> MSQLVLILGDQLSPSIAALDGVDKKQDTIVLCEVMAEASYVGHHKKKIAFIFSAMRHFAEELRGEGYRVRYTRIDDADNAGSFTGEVKRAIDDLTPSRICVTEPGEWRVRSEMDGFAGAFGIQVDIRSDRRFLSSHGEFRNWAAGRKSLT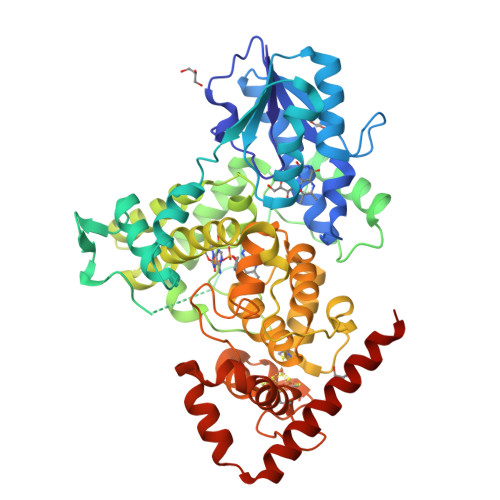MEYFYREMRRKTGLLMNGEQPVGGRWNFDAENRQPARPDLLRPKHPVFAPDKITKEVIDTVERLFPDNFGKLENFGFAVTRTDAERALSAFIDDFLCNFGATQDAMLQDDPNLNHSLLSFYINCGLLDALDVCKAAERAYHEGGAPLNAVEGFIRQIIGWREYMRGIYWLAGPDYVDSNFFENDRSLPVFYWTGKTHMNCMAKVITETIENAYAHHIQRLMITGNFALLAGIDPKAVHRWYLEVYADAYEWVELPNVIGMSQFADGGFLGTKPFAASGNYINRMSDYCDTCRYDPKERLGDNACPFNALYWDFLARNREKLKSNHRLAQPYATWARMSEDVRHDLRAKAAAFLRKLDAAALEHHHHHH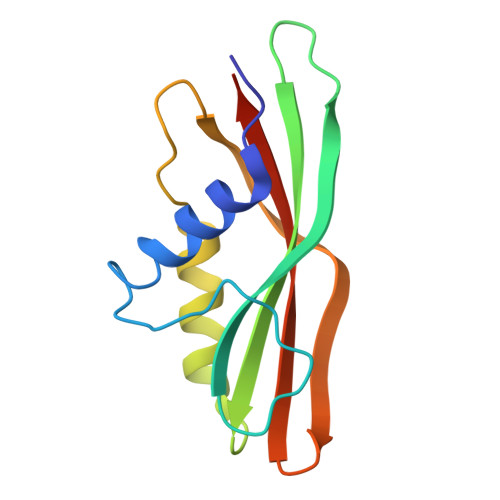> MKSLSFMRVLEAVRTMLEEKGGLDVSIVMRNQVEMPTTMIEMIDQEEEESQTAWKEKYRFAIHHYTNEQDLAGVEMIDTLIQMGFILPEGYKLVAVRHCGKQNLVKENTLIHAKTSFEVSICRELKVKI>[4x]GMLESTKQFLKKYNINDRVLKLYETAMNDIQNQFKILDDIREFNQLKVLNAFQEERISEAHFTNSSGYGYGDIGRDSLDAVYARVFNTESALVRPHFVNGTHALGAALFGNLRPGNTMLSVCGEPYDTLHDVIGITENSNMGSLKEFGINYKQVDLKEDGKPNLEEIEKVLKEDESITLVHIQ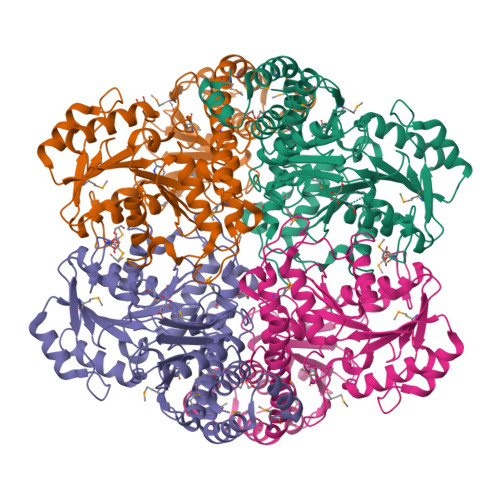RSTGYGWRRALLIEDIKSIVDCVKNIRKDIICFVDNCYGEFMDTKEPTDVGADLIAGSLIKNIGGGIAPTGGYLAGTKDCIEKTSYRLTVPGIGGECGSTFGVVRSMYQGLFLAPHISMEALKGAILCSRIMELAGFEVMPKYDEKRSDIIQSIKFNDKDKLIEFCKGIQTGSPIDSFVSCEPWDMPGYTDQVIMAAGAFIQGSSIELSADAPIREPYIAYLQGGLTFDHAKIGILIALSRIVK>[2x]GSHMLGLIKKKANTLLGIDISSTSVKLLELSRSGGRYKVEAYAVEPLPPNAVVEKNIVELEGVGQALSRVLVKAKTNLKSAVVAVAGSAVITKTIEMEAGLSEDELENQLKIEADQYIPYPLEEVAIDFEVQGLSARNPERVDVLLAACRKENVEVREAALALAGLTAKVVDVEAYALERSYALLSSQLGADTDQLTVAVVDIGATMTTLSVLH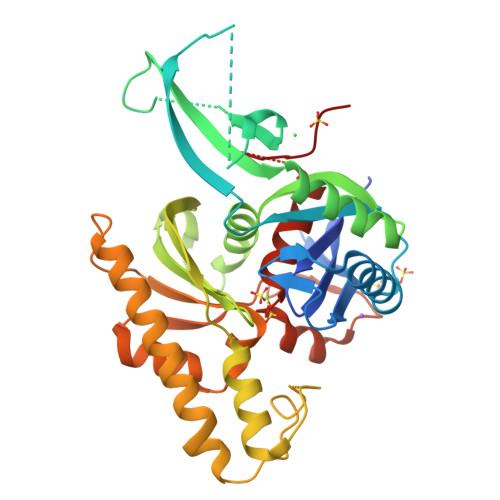NGRTIYTREQLFGGRQLTEEIQRRYGLSVEEAGLAKKQGGLPDDYDSEVLRPFKDAVVQQVSRSLQFFFAAGQFNDVDYIVLAGGTASIQDLDRLIQQKIGTPTLVANPFADMALNGKVNAGALASDAPALMIACGLALRSFDSSGMARINLLPWREE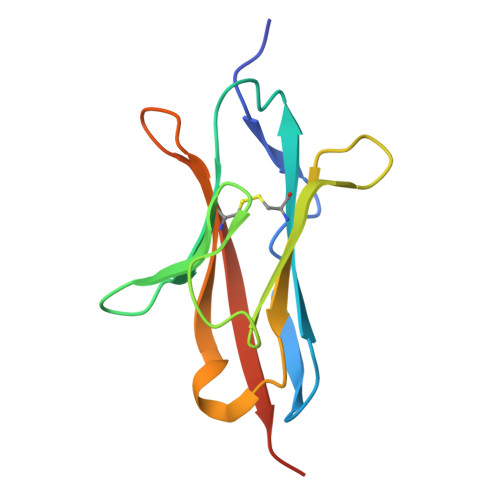> GSGAPPTIQQPSMSSAVALLGQDVDFTCIVNDLGSHMVAFVKADSPPRLLSFDEKVFRRRNKYELKPRIGDLHNEWVLTIKNVQESDRGNYSCQINTEPITLSTGELDVKVPHHHHHH> MSPYSSDTTPCCAAAIARPLPRAHIKEYFYTSGKCSNPAVVFVTRKNRQVCAN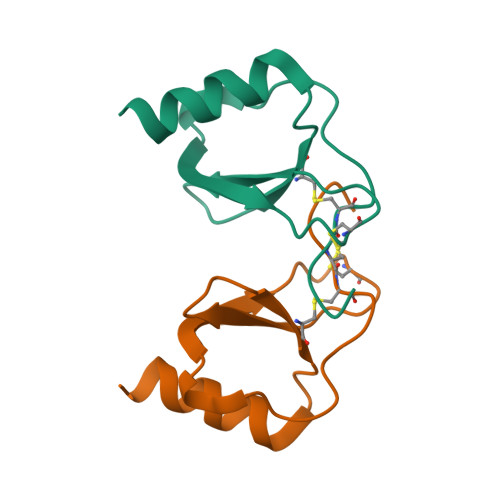PEKKWVREYINSLEMS> GGNSSTSALNSRRNSLDKSSNKQGMSGLPPIFGGESTSYHHDNKIQ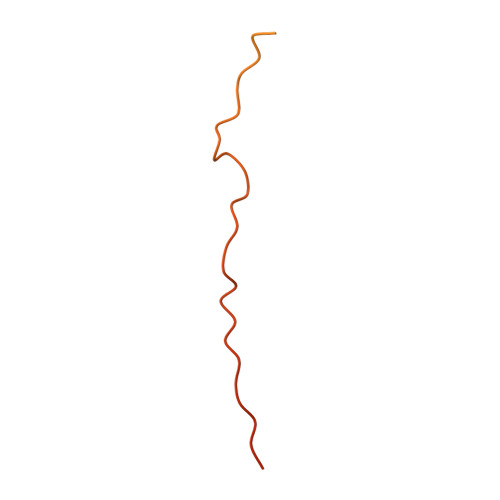KYNQLGVEEDDDDENDRLLNQMGNSATKFKSSISPRSIDSISSSFIKSRIPIRQPYHYSQPTTAPFQAQAKFHKPANKLIDNG> NNVNDLIKVTKQTIKVGDGKDNVAAAHDGKDIEYDTEFTIDNKVKKGDTMTINYDKNVIPSDLTDKNDPIDITDPSGEVIAKGTFDKATKQITYTFTDYVDKYEDIKSRLTLYSYIDKKTVPNETSLNLTFATAGKETSQNVTVDYQDPMVHGDSNIQSIFTKLDEDKQTIEQQIYVNPLKKSATNTKVDIAGSQVDDYGNIKLGNGSTIIDQNTEIKVYKVNSDQQLPQSNRIYDFSQYEDVTSQFDNKKSFSNNVATLDFGDINSAYIIKVVSKY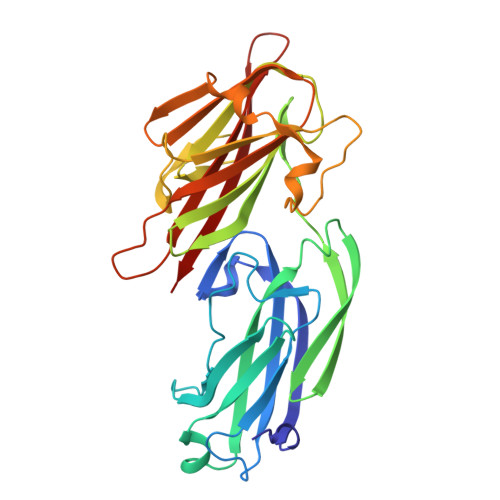TPTSDGELDIAQGTSMRTTDKYGYYNYAGYSNFIVTS The membrane-anchored SNARE (soluble N-ethylmaleimide-sensitive factor acceptor protein receptor) proteins provide the energy to drive membrane fusion in various cellular contexts, such as intracellular trafficking and exocytosis. Supercomplexes of NSF, α-SNAP, and either a syntaxin tetramer or one of two binary complexes of syntaxin—SNAP-25 reveal atomic details of SNARE processing and show how sequential ATP hydrolysis drives disassembly. NSF comprises three structured domains connected by flexible linkers—the adapter N-domain followed by the D1 and D2 AAA+ domains. Six NSF protomers come together to form the active form of the enzyme, a homo-hexamer.

To gain insight into the structural nature of binary complex formation and disassembly by NSF, we prepared a complex of NSF, ɑ-SNAP, and the binary t-SNARE complex (21bin20S) composed of full-length soluble SNAP-25 and soluble syntaxin-1a (1–267) in the absence of divalent cation (i.e., non-hydrolyzing conditions) and performed single-particle cryo-EM. First, models of the NSF D1 and D2 domains with substrate bound in the D1 pore were built into two high-resolution (2.88 Å, 2.92 Å) classes from a single dataset, differing only in the state of F protomer engagement with substrate. Next, the dataset from which they were derived was combined with two additional datasets to enable the 3D reconstruction of weakly populated states with ordered density for the ɑ-SNAP—SNARE spire. Classes with evidence of NSF D1 domains engaging ordered ɑ-SNAP—SNARE sub-complexes were carried forward; eight 21bin20S models were built into reconstructions ranging from 3.39–4.01 Å in resolution, differing mainly in the orientation of N domains and a sub-complex of three ɑ-SNAP molecules and four SNARE motifs relative to the D1 ATPase ring. All classes revealed substrate-bound NSF without Mg2+ needed for ATP hydrolysis and disassembly, and share the same overall architecture, with a spire composed of NSF N-domains and the ɑ-SNAP—SNARE subcomplex on top, the NSF D1 ring in the middle tier, and the NSF D2 ring forming the bottom tier. As such, the stoichiometry of the syntaxin—SNAP-25 complex observed is 2:1, the dominant species in solution. Three ɑ-SNAP molecules bind the 2:1 binary SNARE complex; a flexible linker between SNAP-25 SN1 and SN2 blocks access by a fourth. Of the eight 21bin20S classes with the 2:1 binary SNARE complex from the dataset collected under non-hydrolyzing conditions, six engage syntaxin and two engage SNAP-25 within the pore of the D1 ring. Docking the 2:1 binary complex structure back into the seven individual 21bin20S reconstructions reveals an apparent preference for syntaxin, with six of eight reconstructions featuring the N-terminus of syntaxin H3 bound within the pore of the D1 ring. Taken together, we observe that the NSF D1 ring can bind to at least two different SNAREs, syntaxin, and SNAP-25, in various configurations.

>[6x]GAHMAGRSMQAARCPTDELSLSNCAVVSEKDYQSGQHVIVRTSPNHKYIFTLRTHPSVVPGSVAFSLPQRKWAGLSIGQEIEVALYSFDKAKQCIGTMTIEIDFLQKKNIDSNPYDTDKMAAEFIQQFNNQAFSVGQQLVFSFNDKLFGLLVKDIEAMDPSILKGEPASGKRQKIEVGLVVGNSQVAFEKAENSSLNLIGKAKTKENRQSIINPDWNFEKMGIGGLDKEFSDIFRRAFASRVFPPEIVEQMGCKHVKGILLYGPPGCGKTLLARQIGKMLNAREPKVVNGPEILNKYVGESEANIRKLFADAEEEQRRLGANSGLHIIIFDEIDAICKQRGSMAGSTGVHDTVVNQLLSKIDGVEQLNNILVIGMTNRPDLIDEALLRPGRLEVKMEIGLPDEKGRLQILHIHTARMRGHQLLSADVDIKELAVETKNFSGAELEGLVRAAQSTAMNRHIKASTKVEVDMEKAESLQVTRGDFLASLENDIKPAFGTNQEDYASYIMNGIIKWGDPVTRVLDDGELLVQQTKNSDRTPLVSVLLEGPPHSGKTALAAKIAEESNFPFIKICSPDKMIGFSETAKCQAMKKIFDDAYKSQLSCVVVDDIERLLDYVPIGPRFSNLVLQALLVLLKKAPPQGRKLLIIGTTSRKDVLQEMEMLNAFSTTIHVPNIATGEQLLEALELLGNFKDKERTTIAQQVKGKKVWIGIKKLLMLIEMSLQMDPEYRVRKFLALLREEGASPLDFD;>MKDRTQELRTAKDSDDDDDVTVTVDRDRFMDEFFEQVEEIRGFIDKIAENVEEVKRKHSAILASPNPDEKTKEELEELMSDIKKTANKVRSKLKSIEQSIEQEEGLNRSSADLRIRKTQHSTLSRKFVEVMSEYNATQSDYRERCKGRIQRQLEITGRTTTSEELEDMLESGNPAIFASGIIMDSSISKQALSEIETRHSEIIKLENSIRELHDMFMDMAMLVESQGEMIDRIEYNVEHAVDYVERAVSDTKKAVKYQSKARRKKIM[2x];> MGSSHHHHHHSQDPNSMAEDADMRNELEEMQRRADQLADESLESTRRMLQLVEESKDAGIRTLVMLDEQGEQLERIEEGMDQINKDMKEAEKNLTDLGKFAGLAVAPANKLKSSDAYKKAWGNNQDGVVASQPARVVDEREQMAISGGFIRRVTNDARENEMDENLEQVSGIIGNLRHMALDMGNEIDTQNRQIDRIMEKADSNKTRIDEANQRATKMLGSG;>GMDTSGKQAEAMALLAEAERKVKNSQSFFSGLFGGSSKIEEACEIYARAANMFKMAKNWSAAGNAFCQAAQLHLQLQSKHDAATCFVDAGNAFKKADPQEAINCLMRAIEIYTDMGRFTIAAKHHISIAEIYETELVDVEKAIAHYEQSADYYKGEESNSSANKCLLKVAGYAAQLEQYQKAIDIYEQVGTSAMDSPLLKYSAKDYFFKAALCHFCIDMLNAKLAVQKYEELFPAFSDSRECKLMKKLLEAHEEQNVDSYTESVKEYDSISRLDQWLTTMLLRIKKTIQGDEEDLR[3x]> MTLTTPHPRPEQSESAAQSSLLAGFTPFPAERAQAYRAAGYWRDQLLDSVLRTAARTWPDHIAVIDADHRHTYAELDRLADRAAAGIAGLGIRPGDRVLVQLPNTAEFAVALFGLLRAGAVPVMCLPGHRLAELTHFAEVSSAVALVVADTAGGFDHRDLARELVRSHPDVRHVLVDGDAAEFLSWAEVTRAAPGPVPEIAPDPAAPALLLVSGGTTGAPKLIPRTHQDYVYNATASAELCRLTADDVYLVALPAAHNFPLACPGLLGAMTVGATTVFTTDPSPEAAFAAIDEHGVTATALVPALAKLWAQACAWEPLAPKTLRLLQVGGAKLAAPDAALVRGALTPGLQQVFGMAEGLLNYTRIGDPPEVLENTQGRPLSPDDEIRIVDEVGNEVPPGAEGELLVRGPYTLNGYFNAEAANERSFSPDGFYRSGDRVRRFADGPLAGYLEVTGRIKDVIVRGGENVSALDLEEHLLTHPSVWAAAAVALPDEFLGEKICAVVVFNGPPVSLAELHAHLEQ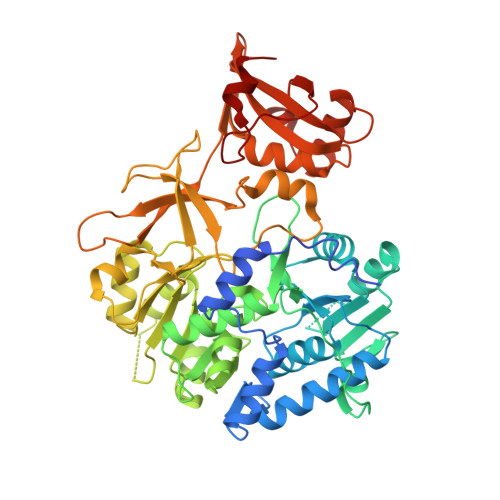RGVAAHSRPDALVPMPSLPTTAVGKIDKKAIVRQLGG>MATSSMSKGCFVFKPNSKKRKISLPIEDYFNKGKNEPEDSKLRFETYQLIWQQMKSENERLQEELNKNLFDNLIEFLQKSHSGFQKNSRDLGGQIKLREIPTAALVLGVNVTDHDLTFGSLTEALQNNVTPYVVSLQAKDCPDMKHFLQKLISQLMDCCVDIKSKEEESVHVTQRKTHYSMDSLSSWYMTVTQKTDPKMLSKKRTTSSQWQSPPVVVILKDMESFATKVLQDFIIISSQHLHEFPLILIFGIATSPIIIHRLLPHAVSSLLCIELFQSLSCKEHLTTVLDKLLLTTQFPFKINEKVLQVLTNIFLYHDFSVQNFIKGLQLSLLEHFYSQPLSVLCCNLPEAKRRINFLSNNQCENIRRLPSFRRYVEKQASEKQVALLTNERYLKEETQLLLENLHVYHMNYFLVLRCLHKFTSSLPKYPLGRQIRELYCTCLEKNIWDSEEYASVLQLLRMLAKDELMTILEKCFKVFKSYCENHLGSTAKRIEEFLAQFQSLDAETKEEEDASGSQPKGLQKTDLYHLQKSLLEMKELRRSKKQTKFEVLRENVVNFIDCLVREYLLPPETQPLHEVVYFSAAHALREHLNAAPRIALHTALNNPYYYLKNEALKSEEGCIPNIAPDICIAYKLHLECSRLINLVDWSEAFATVVTAAEKMDANSATSEEMNEIIHARFIRAVSELELLGFIKPTKQKTDHVARLTWGGC[4x];>MKRDKTSDLVEEYFEAHSSSKVLTSDRTLQKLKRAKLDQQTLRNLLSKVSPSFSAELKQLNQQYEKLFHKWMLQLHLGFNIVLYGLGSKRDLLERFRTTMLQDSIHVVINGFFPGISVKSVLNSITEEVLDHMGTFRSILDQLDWIVNKFKEDSSLELFLLIHNLDSQMLRGEKSQQIIGQLSSLHNIYLIASIDHL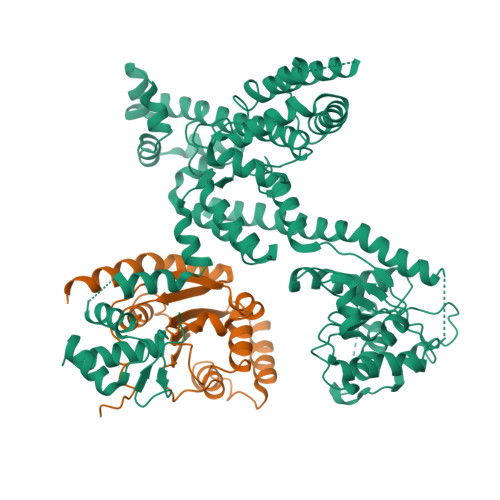NAPLMWDHAKQSLFNWLWYETTTYSPYTEETSYENSLLVKQSGSLPLSSLTHVLRSLTPNARGIFRLLIKYQLDNQDNPSYIGLSFQDFYQQCREAFLVNSDLTLRAQLTEFRDHKLIRTKKGTDGVEYLLIPVDNGTLTDFLEKEEEEA[4x]>[2x]MALTKLVDAGAWQVEVAPAGTVQDSLVFLSPRNFGGVPGTGVDSVAAIEAALAAGDVDLGGEHWFISRPIYCVSGRTIQNGKISTLAAQGSGFMAGSIFAPGNYHPVYVDPVPKLACSS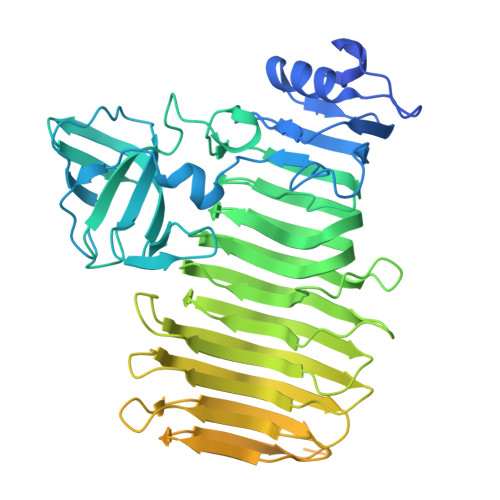TNGSATITVSSHEFVVGDLVRLSSTRGIIGSDAVLVPWYMQLARVVGVSGDTVKLDAPIDTTETLVVHKATPAGYNARFNKPLFVLERATFRNIEVDTWDYWTADSATFECAFEGIRGKARSVVYGNTFCRTNFDNIDITFSNKASEMAFGSHDTNLSNIKFRADSQNWDSTNSVGISWAESGRRCTLDNWQLLVPQGVNLSVLVRISSHRDVQIRKGFIQVHSSSNNILSVEHYGGDRPPCNNILFEDIDVNATGAAAVVVDVYKSANDSAINAVRFEGISYRGATPSVALMRQRGTTSNQVTGVRASLYSANGGAFLVSSAMAWDVRLYGPGLQVPAAVAVLGRTAVLSASRSNLHALRWVTEAIIGVTSTTPGNVLREAVIPAGTLRASDYIDFVISGSTGGATSTKDVLVGVLDSGSNFQGVGFTAPTTEESYYTVQGRISFPTTGNCLITATIGRAGVGVSYARTLVSISNYTTNDVKLQVQAWVGSSAGSLSVQHGCFAPSELTGKGHHHHHH> ADQSFLWNVFQRVDKDRSGVISDTELQQALSNGTWTPFNPVTVRSIISMFDRENKAGVNFSEFTGVWKYITDWQNVFRTYDRDNSGMIDKNE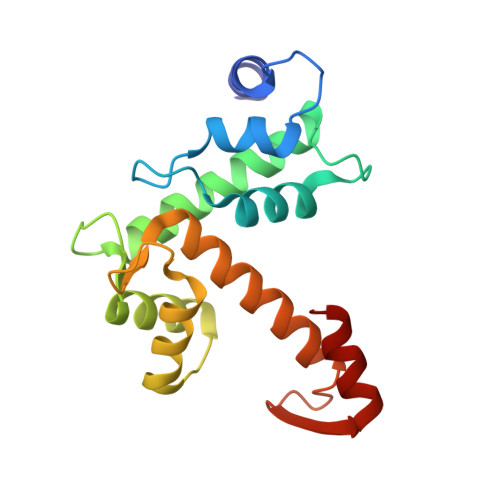LKQALSGFGYRLSDQFHDILIRKFDRQGRGQIAFDDFIQGCIVLQRLTDIFRRYDTDQDGWIQVSYEQYLSMVFSIV> MAAKVFESIGKFGLALAVAGGVVNSALYNVDAGHRAVIFDRFRGVQDIVVGEGTHFLIPWVQKPIIFDCRSRPRNVPVITGSKDLQNVNITLRILFRPVASQLPRIFTSIGEDYDERVLPSITTEILKSVVARFDAGELITQRELVSRQVSDDLTERAATFGLILDDVSLTHLTFGKEFTEAVEAKQVAQQEAERARFVVEKAEQQKKAAIISAEGDSKA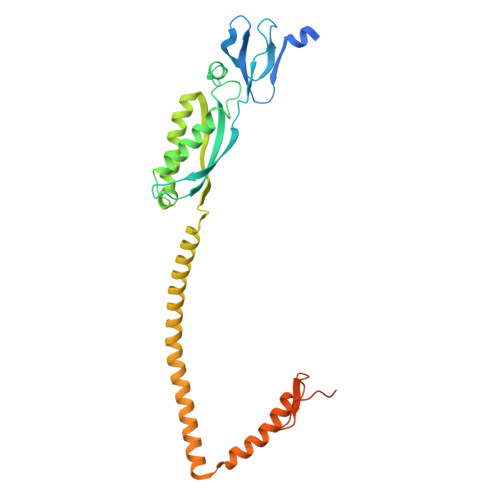AELIANSLATAGDGLIELRKLEAAEDIAYQLSRSRNITYLPAGQSVLLQLPQLEDYKDHDGDYKDHDIDYKDDDDK> PLAAGAVILRRFAFNAAEQLIRDINDVASQ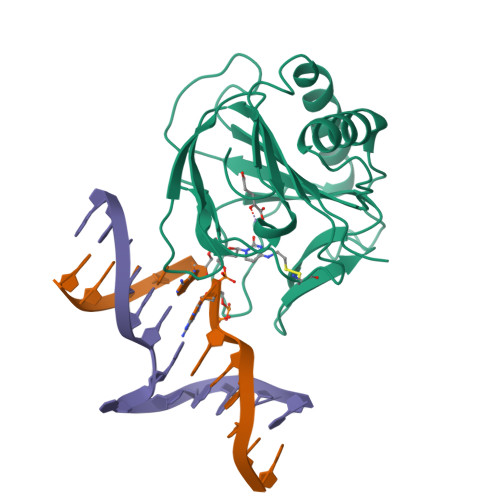SPFRQMVTPGGYTMSVAMTNCGHLGWTTHRQGYLYSPIDPQTNKPWPAMPQSFHNLCQRAATAAGYPDFQPDACLINRYAPGAKLSLHQDKCEPDLRAPIVSVSLGLPAIFQFGGLKRNDPLKRLLLEHGDVVVWGGESRLFYHGIQPLKAGFHPLTIDCRYNLTFRQAGK S-[(2R)-2,3-dihydroxypropyl] (5Z,8Z,11Z,14Z)-icosa-5,8,11,14-tetraenethioate 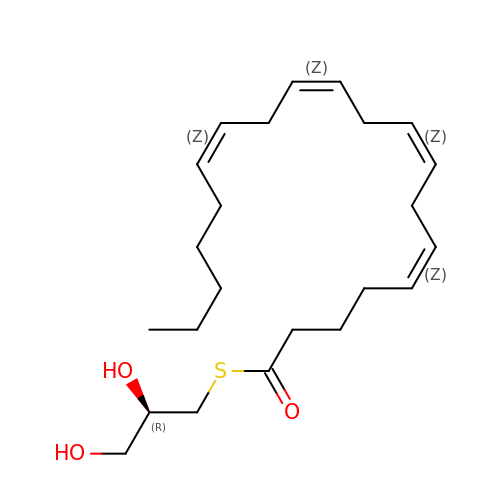| C23 H38 O3 S | UUOPRYPOAXYNLX-NZRYSPDRSA-N> HMLEAKFEEASLFKRIIDGFKDCVQLVNFQCKEDGIIAQAVDDSRVLLVSLEIGVEAFQEYRCDHPVTLGMDLTSLSKILRCGNNTDTLTLIADNTPDSIILLFEDTKKDRIAEYSLKLMDIDADFLKIEELQYDSTLSLPSSEFSKIVRDLSQLSDSINIMITKETIKFVADGDIGGGSVIIKPFVDMEHPETSIKLEMDQPVDLTFGAKYLLDIIKGSSLSDRVGIRLSSEAPALFQFDLKSGFLQFFLAPKFNDEE

Proliferating cell nuclear antigen (PCNA) is a protein that is essential for many DNA metabolic processes including DNA replication, base excision repair, nucleotide excision repair, mismatch repair, and recombination. PCNA is a ring-shaped homo-trimer that acts as a sliding clamp that encircles DNA forming a scaffold for binding numerous proteins involved in DNA metabolism. PCNA is required for translesion synthesis (TLS), which is a pathway for bypassing DNA damage during replication. The subunit interface of PCNA is comprised of two anti-parallel β strands: strand I1 (residues 109 to 117) in domain 1 of one subunit and strand D2 (residues 175 to 183) in domain 2 of the adjacent subunit.

To better understand the role of the subunit interface in translesion synthesis and in other DNA metabolic processes, we used random mutagenesis to generate a series of PCNA mutant proteins with substitutions in either of these two β strands. We first measured the growth rate of these 17 strains in liquid media. Twelve of these strains (A112G, Y114F, S115E, S115G, S115V, S177G, S177L, S177V, G178L, G178M, S178T, and V180A) had slower growth rates than the wild type strain of approximately 4 to 5 hours. The remaining five strains had growth rates similar to the wild type strain of approximately 2 to 3 hours. These data agree reasonably well with the qualitative spotting assay described above in which the A112G, S177G and G178M strains showed minor defects in cell growth and the S115E and G178L strain showed a major defect in cell growth. We next measured the UV sensitivity of these 17 strains. All 17 strains had increased sensitivities to UV radiation to some extent compared to the wild type except G178M. We then examined the rates of spontaneous mutagenesis and the rates of UV-induced mutagenesis of these 17 strains as well as E113G and G178S. By contrast, all 17 strains, except the S177G, S179A, and V180A mutant strains, had statistically significant defects in the rate of UV-induced mutagenesis (with p values less than 0.05). A defect in UV-induced mutagenesis is a characteristic indicator of a defect in error-prone TLS.>SNAMSKLIVPQWPLPKGVAACSSTRIGGVSLPPYDSLNLGAHCGDNPDHVEENRKRLFAAGNLPSKPVWLEQVHGKDVLKLTGEPYASKRADASYSNTPGTVCAVMTADCLPVLFCNRAGTEVAAVHAGWRGLCAGVLEETVSCFADKPENILAWLGPAIGPRAFEVGAEVREAFMAVDAKASAAFIQHGDKYLADIYQLARQRLANVGVEQIFGGDRC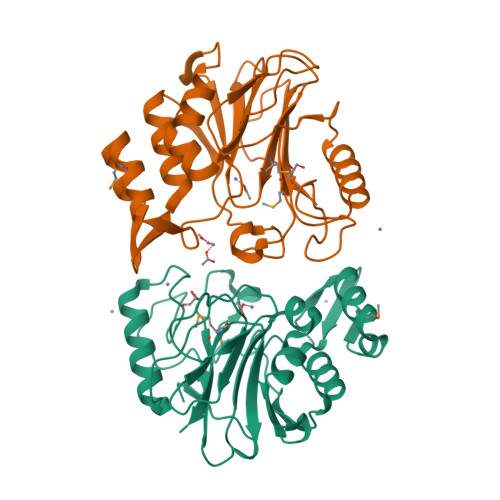TYTENETFFSYRRDKTTGRMASFIWLI[2x]N-methylisoquinolin-1-amine 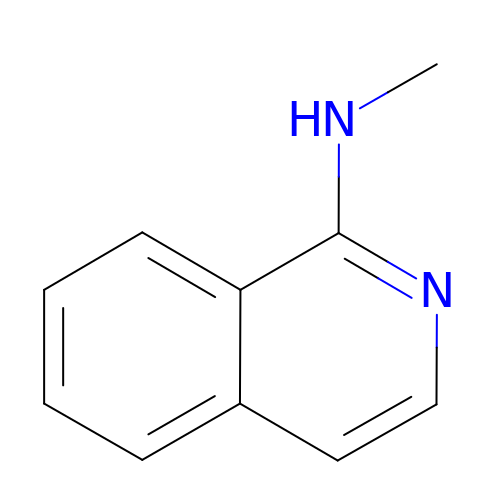| C10 H10 N2 | BILUZSWZYDFPMN-UHFFFAOYSA-N> MDKSSIANKIEAYLGAKSDDSKIDQSLKADPSEVQYYGSGGDGYYLRKNICKITVNHSDSGTNDPCDRIPPPYGDNDQWKCAIILSKVSEKPENVFVPPRRQRMCINNLEKLNVDKIRDKHAFLADVLLTARNEGERIVQNHPDTNSSNVCNALERSFADIADIIRGTDLWKGTNSNLEQNLKQMFAKIRENDKVLQDKYPKDQNYRKLREDWWNANRQKVWEVITCGARSNDLLIKRGWRTSGKSNGDNKLELCRKCGHYEEKVPTKLDYVPQFLRWLTEWIEDFYREKQNLIDDMERHREECTSEDHKSKEGTSYCSTCKDKCKKYCECVKKWKSEWENQKNKYTELYQQNKNETSQKNTSRYDDYVKDFFKKLEANYSSLENYIKGDPYFAEYATKLSFILNSSDANNPSEKIQKNNDEVCNCNESGIASVEQEQISDPSSNKTCITHSSIKANKKKVCKHVKLGVRENDKDLRVCVIEHTSLSGVENCCCQDFLRILQENCSDNKSGSSSNGSCNNKNQEACEKNLEKVLASLTNCYKCDKCKSEQSKKNNKNWIWKKSSGKEGGLQKEYANTIGLPPRTQSLCLVVCLDEKGKKTQELKNIRTNSELLKEWIIAAFHEGKNLKPSHEKKNDDNGKKLCKALEYSFADYGDLIKGTSIWDNEYTKDLELNLQKIFGKLFRKYIKKNNTAEQDTSYSSLDELRESWWNTNKKYIWLAMKHGAGMNSTTCCGDGSVTGSGSSCDDIPTIDLIPQYLRFLQEWVEHFCKQRQEKVKPVIENCKSCKESGGTCNGECKTECKNKCEVYKKFIEDCKGGDGTAGSSWVKRWDQIYKRYSKYIEDAKRNRKAGTKNCGPSSTTNAAENKCVQSDIDSFFKHLIDIGLTTPSSYLSIVLDDNICGADKAPWTTYTTYTTTEKCNKETDKSKLQQCNTAVVVNVPSPLGNTPHGYKYACQCKIPTNEETCDDRKEYMNQWSCGSARTMKRGYKNDNYELCKYNGVDVKPTTVRSNSSKLDDKDVTFFNLFEQWNKEIQYQIEQYMTNTKISCNNEKNVLSRVSDEAAQPKFSDNERDRNSITHEDKNCKEKCKCYSLWIEKINDQWDKQKDNYNKFQRKQIYDANKGSQNKKVVSLSNFLFFSCWEEYIQKYFNGDWSKIKNIGSDTFEFLIKKCGNDSGDGETIFSEKLNNAEKKCKENESTNNKMKSSETSCDCSEPIYIRGCQPKIYDGKIFPGKGGEKQWICKDTIIHGDTNGACIPPRT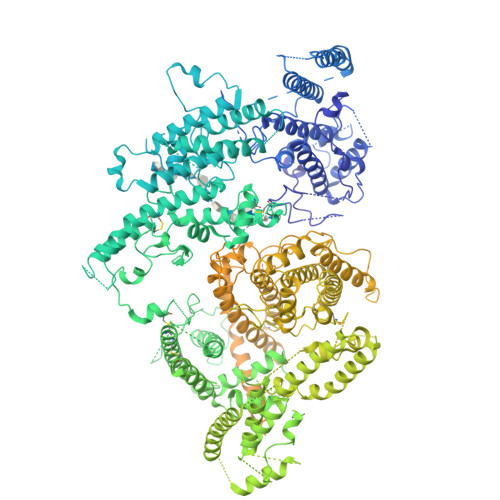QNLCVGELWDKRYGGRSNIKNDTKESLKQKIKNAIQKETELLYEYHDKGTAIISRNPMKGQKEKEEKNNDSNGLPKGFCHAVQRSFIDYKNMILGTSVNIYEYIGKLQEDIKKIIEKGTTKQNGKTVGSGAENVNAWWKGIEGEMWDAVRCAITKINKKQKKNGTFSIDECGIFPPTGNDEDQSVSWFKEWSEQFCIERLQYEKNIRDACTNNGQGDKIQGDCKRKCEEYKKYISEKKQEWDKQKTKYENKYVGKSASDLLKENYPECISANFDFIFNDNIEYKTYYPYGDYSSICSCEQVKYYEYNNAEKKNNKSLCHEKGNDRTWSKKYIKKLENGRTLEGVYVPPRRQQLCLYELFPIIIKNKNDITNAKKELLETLQIVAEREAYYLWKQYHAHNDTTYLAHKKACCAIRGSFYDLEDIIKGNDLVHDEYTKYIDSKLNEIFDSSNKNDIETKRARTDWWENEAIAVPNITGANKSDPKTIRQLVWDAMQSGVRKAIDEEKEKKKPNENFPPCMGVQHIGIAKPQFIRWLEEWTNEFCEKYTKYFEDMKSNCNLRKGADDCDDNSNIECKKACANYTNWLNPKRIEWNGMSNYYNKIYRKSNKESEDGKDYSMIMEPTVIDYLNKRCNGEINGNYICCSCKNIGENSTSGTVNKKLQKKETQCEDNKGPLDLMNKVLNKMDPKYSEHKMKCTEVYLEHVEEQLKEIDNAIKDYKLYPLDRCFDDKSKMKVCDLIGDAIGCKHKTKLDELDEWNDVDMRDPYNKYKGVLIPPRRRQLCFSRIVRGPANLRNLKEFKEEILKGAQSEGKFLGNYYNEDKDKEKALEAMKNSFYDYEYIIKGSDMLTNIQFKDIKRKLDRLLEKETNNTEKVDDWWETNKKSIWNAMLCGYKKSGNKIIDPSWCTIPTTETPPQFLRWIKEWGTNVCIQKEEHKEYVKSKCSNVTNLGAQESESKNCTSEIKKYQEWSRKRSIQWEAISEGYKKYKGMDEFKNTFKNIKEPDANEPNANEYLKKHCSKCPCGFNDMQEITKYTNIGNEAFKQIKEQVDIPAELEDVIYRLKHHEYDKGNDYICNKYKNINVNMKKNNDDTWTDLVKNSSDINKGVLLPPRRKNLFLKIDESDICKYKRDPKLFKDFIYSSAISEVERLKKVYGEAKTKVVHAMKYSFADIGSIIKGDDMMENNSSDKIGKILGDGVGQNEKRKKWWDMNKYHIWESMLCGYKHAYGNISENDRKMLDIPNNDDEHQFLRWFQEWTENFCTKRNELYENMVTACNSAKCNTSNGSVDKKECTEACKNYSNFILIKKKEYQSLNSQYDMNYKETKAEKKESPEYFKDKCNGECSCLSEYFKDETRWKNPYETLDDTEVKNN>GSHMRLRSVSDKNSSALLETGSLLHSPFDEEQQILKKKAEEVKPYLNGRSMYLVGMMGSGKTTVGKIMARSLGYTFFDCDTLIEQAMKGTSVAEIFEHFGESVFREKETEALKKLSLMYHQVVVSTGGGAVIRPINWKYMHKGISIWLDVPLEALAHRIAAVGTGSRPLLHDDESGDTYTAALNRLSTIWDARGEAYTKASARVSLENITLKLGYRSVSDLTPAEIAIEAFEQVQS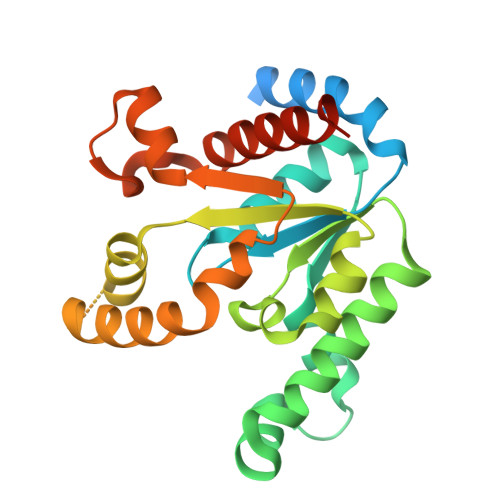YLEKEDGMARPDGL[2x]> MKISVSKNDLENALRYLQAFLDKKDASSIASHIHLEVIKEKLFLKASDSDIGLKSYIFTQSSDKEGVGTINGKKFLD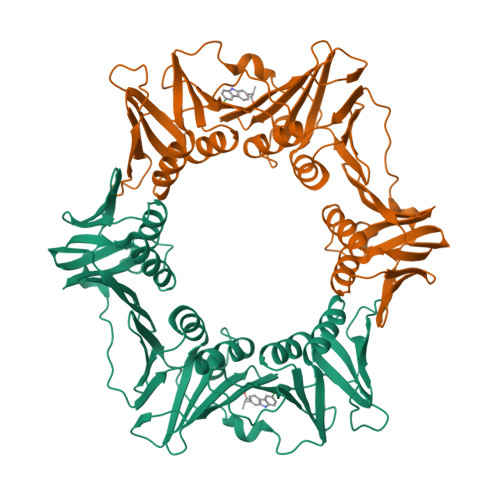IISCLKDSNIILETKDDSLAIKQNKSSFKLPMFDADEFPEFPVIDPKVSIEVNAPFLVDAFKKIAPVIEQTSHKRELAGILMQFDQKHQTLSVVGTDTKRLSYTQLEKISIHSTEEDISCILPKRALLEILKLFYENFSFKSDGMLAVIENEMHTFFTKLIDGNYPDYQKILPKEYISSFTLGKEEFKESIKLCSSLSSTIKLTLEKNNALFESLDSEHSETAKTSVEIEKGLDIEKAFHLGVNAKFFLEALNALGTTQFVLRCNEPSSPFLIQESLDEKQSHLNAKISTLMMPITL>[2x]GGSMATNENLPEIMTKLWDSKAQGEQEELHLLKGSDCNLTIDITEKCLRLAQRSAYQLHTETSATKRIQKFFLLGSLNINKDDRVIINIDRFDPGRIIDRKEGNKSLHVPTAVIPGDVIIPLSMQLACLGSEGVSPFSISEYYDAFQTLTKNLKLSCDSVDIKDMLSL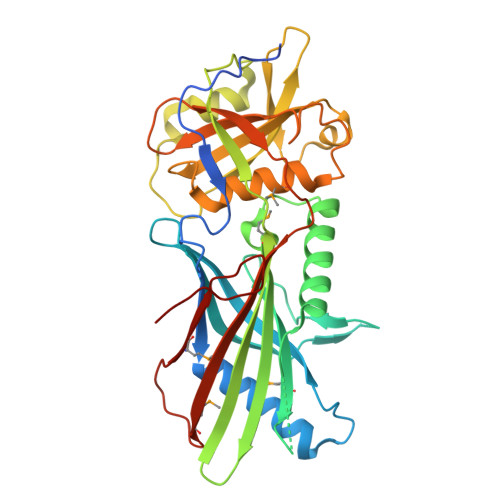KIHATYYVDSDEISINVTSGVVVPSALITAVPILPVSIVPTALARSLSGPLHLSNFQDTQKSGYVAINNSHNLLLVLDSDPKLSSIPLVGIWVDGVISIHHPYVWSACMRYLYSQRLTNKIRDGSTGFILVLYTQTRPKPEFWECSFSGKSDKFLYCQASDDIFMEKVAKTRNEYMRLQLVPNEFGENLYFQ> YSYTEKKRIRKDFGKRPQVLDVPYLLSIQLDSFQKFIEQDPEGQYGLEAAFRSVFPIQSYSGNSELQYVSYRLGEPVFDVQECQIRGVTYSAPLRVKLRLVIYEREAPEGTVKDIKEQEVYMGEIPLMTDNGTFVINGTERVIVSQLHRSPGVFFDSDKGKTHSSGKVLYNARIIPYRGSWLDFEFDPKDNLFVRIDRRRKLPATIILRALNYTTEQILDLFFEKVIFEIRDNKLQMELVPERLRGETASFDIEANGKVYVEKGRRITARHIRQLEKDDVKLIEVPVEYIAGKVVAKDYIDESTGELICAANMELSLDLLAKLSQSGHKRIETLFTNDLDHGPYISETLRVDPTNDRLSALVEIYRMMRPGEPPTREAAESLFENLFFSEDRYDLSAVGRMKFNRSLLREEIEGSGILSKDDIIDVMKKLIDIRNGKGEVDDIDHLGNRRIRSVGEMAENQFRVGLVRVERAVKERLSLGDLDTLMPQDMINAKPISAAVKEFFGSSQLSQFMDQNNPLSEITHKRRISALGPGGLTRERAGFEVRDVHPTHYGRVCPIETPEGPNIGLINSLSVYAQTNEYGFLETPYRKVTDGVVTDEIHYLSAIEEGNYVIAQANSNLDEEGHFVEDLVTCRSKGESSLFSRDQVDYMDVSTQQVVSVGASLIPFLEHDDANRALMGANMQRQAVPTLRADKPLVGTGMERAVAVDSGVTAVAKRGGVVQYVDASRIVIKVNEDEMYPGEAGIDIYNLTKYTRSNQNTCINQMPCVSLGEPVERGDVLADGPSTDLGELALGQNMRVAFMPWNGYNFEDSILVSERVVQEDRFTTIHIQELACVSRDTKLGPEEITADIPNVGEAALSKLDESGIVYIGAEVTGGDILVGKVTPKGETQLTPEEKLLRAIFGEKASDVKDSSLRVPNGVSGTVIDVQVFTRDGVEKDKRALEIEEMQLKQAKKDLSEELQILEAGLFSRIRAVLVAGGVEAEKLDKLPRDRWLELG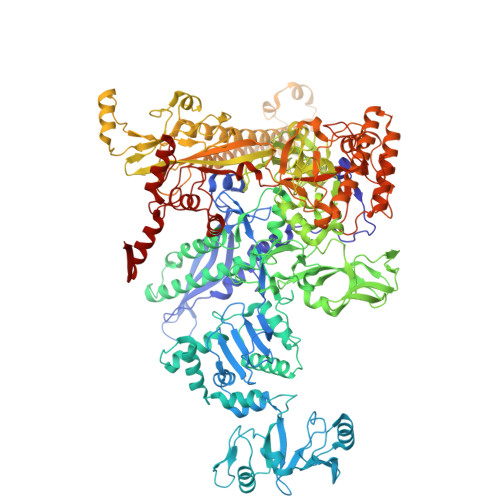LTDEEKQNQLEQLAEQYDELKHEFEKKLEAKRRKITQGDDLAPGVLKIVKVYLAVKRRIQPGDKMAGRHGNKGVISKINPIEDMPYDENGTPVDIVLNPLGVPSRMNIGQILETHLGMAAKGIGDKINAMLKQQQEVAKLREFIQRAYDLGADVRQKVDLSTFSDEEVMRLAENLRKGMPIATPVFDGAKEAEIKELLKLGDLPTSGQIRLYDGRTGEQFERPVTVGYMYMLKLNHLVDDKMHARSTGSYSLVTQQPLGGKAQFGGQRFGEMEVWALEAYGAAYTLQEMLTVKSDDVNGRTKMYKNIVDGNHQMEPGMPESFNVLLKEIRSLGINIELEDE We identify the core polyadenylation complex within T. gondii and establish CPSF4 as a reader for m6A-modified mRNAs, via a YTH domain within its C-terminus, a feature which is shared with plants. In the CPSF complex, the T. gondii CPSF4 subunit can be distinguished as one holding a unique architecture which interestingly is shared with the plant CPSF30L family, and it constitutes a co-occurrence of three zinc fingers and a conserved YTH domain. Overall, the CPSF4 YTH domain folds into a well-structured domain featuring six alpha helices (α1–6) and five beta sheets (β1–5). In parallel to the orthodox 3’end processing mechanism which occurs independently of the m6A modification, we propose the existence in T. gondii of an m6A-dependent polyadenylation through which the m6A site would guide the polyadenylation machinery, via the ability of the CPSF4 YTH to bind this modification, thus allowing the recognition of the respective m6A-dependent polyadenylation site, and the proper termination at a relevant locus.

To validate the biochemical function of the YTH domain contained within CPSF4 (predicted from residues 434 to 598), we undertook to recombinantly express the domain in E. coli with an N-terminal TEV cleavable 8*His tag with minimized extremities so as to limit disordered regions and obtained pure and monodisperse preparation of the protein. TgCPSF4-YTH (aa 434–598), as used in the ITC experiments generated distinct crystal forms: Apo, m6A bound and m6A modified 7-mer RNA bound which all diffracted to high resolutions (up to 1.45 Å for the RNA bound form), sometimes using fully automated upstream crystal harvesting (using the EMBL crystal direct technology) and automated crystal diffraction (using MASSIF-1 at the ESRF). The binding of m6A favors crystal growth in P1 symmetry instead of a P41212 symmetry, however, the binding event does not induce important conformational changes within the protein, the N-terminal residues (ranging from 437 to 446) fold as random coils on opposite sides, most likely as a consequence of crystal packing. (C) Cartoon and stick superposition of the m6A-bound CPSF-4 YTH (green/yellow/blue) against the apo form (white) visualized in UCSF Chimera.

> GDPFGHVASPQSTKRFFIIKSNRMSNIYTSIQHGVWATSKGNSRKLSNAFTSTDHVLLLFSANESGGFQGFGRMMSLPDPQLFPGIWGPVQLRLGSNFRVMWLKQCKIEFEELGKVTNPWNDDLPLRKSRDGTEVPPALGSLLCTWMSQRPSEDLLAGTGIDPATR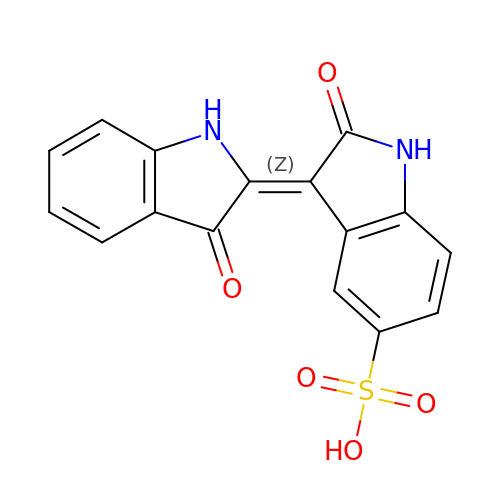2',3-DIOXO-1,1',2',3-TETRAHYDRO-2,3'-BIINDOLE-5'-SULFONIC ACID | C16 H10 N2 O5 S | IHBOEHLUIBMBMY-YPKPFQOOSA-N> ATIKDVAKRANVSTTTVSHVINKTRFVAEETRNAVWAAIKELHYSPSAVARSLKVNHTKSIGLLATSSEAAYFAEIIEAVEKNCFQKGYTLILGNAWNNLEKQRAYLSMMAQKRVDGLLVMCSEYPEPLLAMLEEYRHIPMVVMDWGEAKADFTDA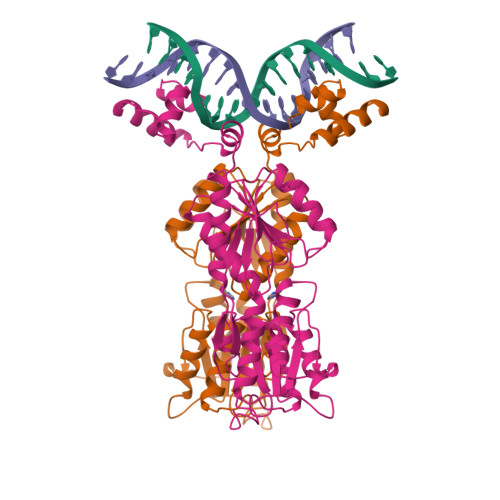VIDNAFEGGYMAGRYLIERGHREIGVIPGPLEANTGAGRLAGFMKAMEEAMIKVPESWIVQGDFEPESGYRAMQQILSQPHRPTAVFCGGDIMAMGALCAADEMGLRVPQDVSLIGYDNVRNARYFTPALTTIHQPKDSLGETAFNMLLDRIVNKREEPQSIEVHPRLIERRSVADGPFRDYRR>NTKYNKEFLLYLAGFVDGDGSIIAQIKPNQSYKFKHQLSLTFQVTQKTQRRWFLDKLVDEIGVGYVRDRGSVSNYILSEIKPLHNFLTQLQPFLKLKQKQANLVLKIIEQLPSAKESPDKFLEVCTWVDQIAALNDSKTRKTTSETVRAVLDAA[2x]

I-CreI is a homodimeric member of LHEs family, which recognizes and cleaves a 22 bp pseudo-palindromic target (5′- CAAAACGTCGTGAGACAGTTTG -3′). Each I-CreI monomer binds its own DNA target region generating the catalytic centre at the dimer interface. This region contains two catalytic aspartic acids (D20, one per each monomer). The aspartic side chains participate in the cleavage of the DNA strands along the minor groove, resulting in the hydrolysis of specific phosphodiester bonds upon the coordination of three divalent metal ions.

To decipher why a G at this position restricts cleavage, we made DNA substitutions in the cleavable DNA target to render it non-cleavable. For this purpose, we exchanged GT in positions −5 and −4 of the wild type coding strand target (I-CreI_D75N_target, Fig. 1b upper sequence) by TG, generating the non-cleavable target I-CreI_D75N_target-null (Fig. 1b bottom sequence). As expected from in vitro cleavage experiments, the comparison of the crystal structures of the I-CreI variants in complex with its cleavable and non-cleavable target DNAs in favourable catalytic conditions (2 mM Mg2+), showed the hydrolysed phosphodiesters in the cleavable targets while the non-cleavable targets displayed the intact phosphodiester bonds. We observed that the structures of the variants in complex with the cleavable targets showed the presence of the 3 reported catalytic ions, while the structures in complex with the non-cleavable targets indicated the presence of just 2 catalytic ions, with the central metal position occupied by a water molecule. The absence of the central metal ion in the non-cleaved structures, would explain the different catalytic behaviour. Our results clearly point out that in the cases of I-CreI_D75N_target-null and I-CreI_3115_target-null sequences bound to the I-CreI_D75N and I-CreI_3115 proteins, A at position +1 largely deviates with respect to the usual B-DNA conformation. In particular, we found that in ~ 30% (I-CreI_D75N_target-null) and ~ 60% (I-CreI_3115_target-null) of the simulation time A +1 is not paired and is found stacked to the corresponding nucleobases. The larger flexibility of the A +1 in the active centre explains the low occupancy of the central metal ion within the active site, disturbing the positioning of the P-O bond for catalysis, thus inhibiting cleavage.> MLRSRIPCVVVTLVQCRAMHGKPTQSHKVRTQHSRRWWTQSKARHLTAMPHDEC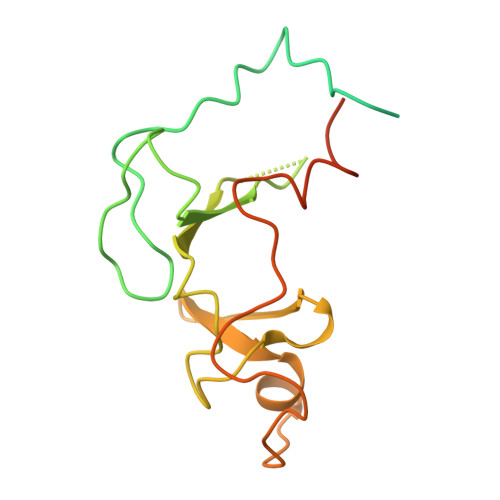KSRPHFPAYNEDVDRPMVVPPDAICFNCDKPIDAGDVNSYVWIPAGNATVPTPQGYFFHFGCFKCNRCKYRLGHNKFYSKDGKAWCIPCALGRDVRVPTRRWHTSYVNTHRTGSRLTGHFFPRHSHQMEFLFDPNS> LPTSNPAQELEARQLERTTRDDLINGNSASCADVIFIYARGSTEAGNLGTLGPSIASNLESAFGKDGVWIQGVGGAYRATLGDNALPRGTSSAAIREMLGLFQQANTKCPDATLIAGGYSQGAALAAASIEDLDS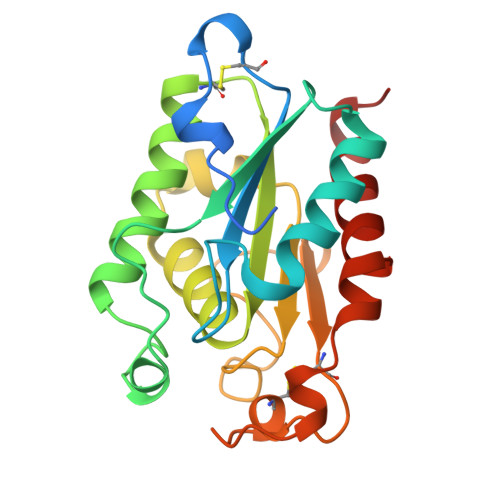AIRDKIAGTVLFGYTKNLQNRGRIPNYPADRTKVFCNTGDLVCTGSLIVAAPHLAYGPDARGPAPEFLIEKVRAVRGSA{4-[2,2-BIS(5-METHYL-1,2,4-OXADIAZOL-3-YL)-3-PHENYLPROPYL]PHENYL}SULFAMIC 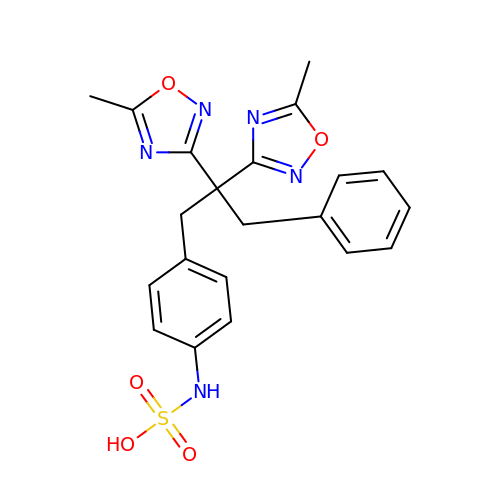ACID | C21 H21 N5 O5 S | SXDBFKLPNPUPRI-UHFFFAOYSA-N> MGDHSQKDSPEDFIINRLSQALGIQKEKIKKSLETQQDDKGEVTNKDEFQGFIQQDNSTNILWVSGQSEKCTFYYGQLPPIDKFKKKGIAVIKLGLHKLTNENVAKDVVVVEITNNLLEHLNSVFNEIMSPVMQNPLNQQGWTDLVAKDLMEKFNNYVAQVYVLLGQIKGKTMLPLPSHKLTSSDTTPDKDKAHVFEGSIITWTKQIKNVLKLEPEQLLKYGNDPGPLAEIEFWQNKRDNLNLIDSQLKSVEVQNILHFLDNNKSTYTTPFTKLQAEVKKARLEANENYRYLFTLKDLFSKLQESQPSDFPTLYELFIPIMHTILLIYNKSKTYNQPPRLVVLIREICNAIISNAQAFVDKDTIFSLIDSKETTEACDKLQVTLDVCSKFKDAYFEYKAKAGGNWKLTSNALFVRLDSFLERCQDILHLTNTIVQFNKLEKIELGGTKGKTLTESIAQIFKEFEEAVQAFTSVSYDIMNIAEKKFDDDFYEFRSKIKELERRLASVITQGFDDYDTIYGRFKLLDNFEGLLTRPIIADELEKKHIVLLEMYKQDLKQVQSIFLEGKQFVDSMHENAPLFLNMPPIAGALTWCKSLRDRIQEPIEKLAQLGQGITEREEYKDVQKLYTSITKSIKDYEDQKILSWEKEVEDSSQDKLKQTLLCKDENDLIKVNFDPSLVRLLKEVKYFLLLRLEVPTTAKDIYTKAETYRTQIVALDMIVDNYNHIKTCLLPVEEPLVKKKIQDMEEEVKPGIEEIRWKSTNIDQFISKSKSIVDQLFETVNKMKDSLQKIHKSLANFNVKIIERKNRPMSPDDYDQFLKAIFSNKLTIVKDNGNQIQKLVKEVLDAVKADKKQNSWKNYNDYVNVIVIEGISTAIQTALLHLNEQINPVFIKRNDISPLFDIRLELGQSGIQFDPEIGESSNQLTVRNTIRNWINDFFNIAGTIQRLDTTMPGDFLQEIRSFFEIKQCLAMITQNLEWIENECNQFRARFDTYSYLWTEDEQISFNRFLDENEPKDEDGKGGDDDEGENTEKQNPLLKGCRAKIPNLDLFDEKITHLKAIQQEISRIKTPEDISWLRINLQPMKTALDARVTRWIRVYTDFLVNQFRTTQKNLLDFIEKTKDGIKKNPADHENLHDKKLLMSVMKVISDVKDVEPRREGIITRMKEMVTKLKKHNVPITEKGTDDPLQQIDNANSNFIEIYGRVFKVKADIIPLQAEETQNIKRDLDIFMKEVESFRKEFMQKLPFDYTESMGYENINNAYDTIMVYYHKLTAIEGRALEYNNLEKLFELQKSNYKQLKDCMNDLKNLKTMWDAIALIHFQYNDWKTKPWRQIKADILLDTNKTLGTQIKNLPKEIRNFKGYNVIVEKVKNMGTVLPLVSALHSEFMEDRHWSQLKQITGTVFDHNSLSFYFEDILALNLYKYENTVNEIVDVAQKEAKIEKKLKNIEQWWSKQVFEFTEYKETKTFASLDNMMEVLDQHSLDLMGMKSQGKYVEFFYDRVEDWREKLGRVDVVVNEWLKVQKNWKILYNIFLLSEDIRMQLPEDTKVFEGVDKEFKDMMSEVSANPSVVEACTIERRDVLVGWSQAIKKCEKALNDYLEQKKKSFPRFYFLSNQSLLTILSNGQNAPKVCEYLGDCFDGLKTLTFEPPANPAETSKVGIGMISKDDEKVPFSSKFICEGAVEHWLLNLEFRMRETLQEILEGAKNTADLWDSGDKPREEWVEGYNAQIALLTTTIVWTEDVGRAFEDLAGGSETAMKECQKLIEVRLENLIKKVRGDLHILERWKIINIITIDVHSRDVVEKFVIQKVSEAESFAWLSQLKFYWENKPDSDMHLRQTLRFPWEKDKNKNKCIIRIVDWFRFYSYEYIGNAIRLVITPLTDRCYITLTQALNLTMGGAPAGPAGTGKTETTKDLGRAIGIPVMVFNCSDQMNKDSMAQIFMGLSQSGAWGCFDEFNRISIEVLSVVSTQVKCVLDALKEKKTKFSFVEEGEIQLQDTVGFFITMNPGYAGRTELPENLKALFRSCAMVVPDLALICENMLM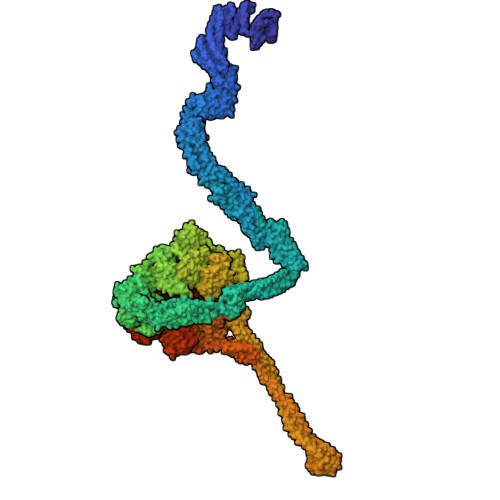SEGFTMARVLSRKFVSLYMLSRELLSKQKHYDWGLRAVKSVLRQAGKLKRGDPDMPEDPLLMRALRDFNMPKIVTDDKVIFRRLIGDLFPKLDPPTKQNPELKKIVQDTTKKDMGLVAEELFVTKVVQLAEILEVRHCCFVIGPPGSGKTCVWKTLIKSYINSGEDAEYDTLNPKAVTSDELFGAYTKTKEWKNGVIAVIMKNQVKNEEKYKATHMHKWSVLDGDIDPEWIESLNTVMDDNKVLTLVSNDRIFLTPQMRLIFEISNLRNATPATVSRAGVLFINETDIGWMPYMNSWLERSQINILKQQKEMANMPEYPVIDDVAKSVFYRCFQSYFEQNIDVHDKNRVRHICPMVDIAMIQTICTILDALLIQHLPKLKQMKEEDEKQALEAFFIFAGLWAIGGPVGGGQDDSKDMKEFNTVWKGAAKVKFPEQGLCYDYYYDINENKWNTWKVEDYLPNDQPLFSKIYVATIHTTRLRYMIDIHLQRRKPILFIGSAGTGKTAVVRDYLNSTRPEQVSHKTINFSSFTDSLALQKNIESMVEKKNGRNYGSATNKVLICFIDDFNMPYVDKYGTQSPIQLLRLILDYGSIFNREQLEERKFLQDLLFFGCLNQKSGSFTVDLRLQRNFSVFSMYTPSSDVIKTIFGSILNAHLSTIDDKAQKMAFKLVEATYFTFDKILKNTTAFAPSAKRFHYQFNFRELARVCEGICRTTPGQYSGGDQGKLVRLWAHEMKRTFEDRFIANEHVEFFRRYLTEAISKCIGEFPETENPIAEPLIFTGFVAAHQGLDQQYTQCTIPVLKRVLDDKLEEYNEVKAQMNLVLFQQAMEHVSRICRILDMPGNNALLVGVGGSGKQSLCRLSTFINGFEIDQLVVTASFTINDLRNNLQEIYKKIAKPNSIARVFMITDSQIKEEQFLIPINDMLNSGWIFDLFPKEDMDSLVSGVRNEAKGEGVDVNNLTALTSYFLDKIRKNLKVVLCFSPVGDTMRIRSRKFPGIINNTSIDWFHPWPHEALIDVAFRFLEEIEFPTEEIRQSISLNMAKVHSSIDTANEKFLKLERRYNYTTPKSFLELIDFYKKLLTEKRETIQRQIQRYEMGLNILAETQNKVQGLQEELKVKMVEVNKQREETDILIEKVGKESALAEEEQTIANAEEEKTNVAAAEAEKISKEATEALAEALPALRSAEAAVDCLKKPHVTEMKNLGSPPAGVIVTARVVLILFNQGITLNDPDEKVWKKAVTFMNNPQAFIDKVKSFDGENIEPNIIEQSNKIIQDPSKKFNEKDMAGQSYAASKLCAWAVNIVTFNKIFKQVKPLQDAQKQANEILEEKKKELAIVKQRVAELNARVNSLKRQLEEAEARKMIVEQDAARCQSRLSAAENLVNGLAGENKRWTQNVKFLKENIKSMIGDSLLASAFVSYIGAFSAKLRLELWKNTWLPDIIEKGIPITEGIEPLKILTTEAIKSKWKNEGLPADPMSLENAAIITACARWPLIIDPQLQGSTWIRGKQGENLTTISLSQPKWLGALTSSISSGRAVLIEGIQQEIDATLDPLLQRAVKKNGNQLQLEIGGDPIDYDPNFKLFLMTKLINPHFRPEIAAQCTIINFIVTESGLEEQFIAMVVNIEKNELEMAKQDLVKKQNEYAVTLDKLESDLLQSLSEADPATILDNTELIQNLDKTKKTTIEITEQQQKAKVTEAEINIQREHYRVVAAEGSMLYFLVISLSVMDHMYQYSLESFITFFFKAINRTTVRDENRIPTLILNIRQTIYQWISRGLFEKHKLIFLTLIVFRLMQKKIIDVAYEVAEMDFLIKCPARPGVENTLDWLPNISWDQIQGLINLEEFRNFAHQLEKEAPNRFKDWYNELQPEDQKLPLDWKRLDSMPFKKLLVLRCLRPDRMTISLNNFIRAVLPQGDAFVEMDQKLAFSEILESVINEDSESTIPIFFILSPGSDPVKEVEKIAKKKRIEPGKNFFNIALGQGQDEIARRRIEEGNKEGHWVMLQNIHLMPTWLIELEKILDSYSGEAGGGNSEFRLFLSAEPSTGIPIGILDRSIKLTNEPPAGLKANMKRAWTYFSKEEIEDKDPKIKSILFALCFFHSTLIERRRFGPKGWNMSYPFNMGDLRDSYLVMNRYMEQNQGGKVPFNDLIYIFGEIMYGGHIVDDWDRRLCNSYLFNTMHEQLFDELELFPYIEGKGLSFKVPGQNPYEKYIEHIETSLKQETPLAYGLHPNAEIGFRTDQCKTLFNTLLELMPKEQSRDEKSSDIKSSNEMASDLIKQLLEDSELKNKIFNMEEIKNKIDAENKGPYQNVFLQEIEYMNALLSEIVKDLEEIGQGLSGLLTVSENMEMIIESIALSRVPASWQKLAYPSKRGLQSWLANLFQRIEQLNIFRDDPYSIPRVVMISRFFNPQSFLTAIMQVISRAKAYELNKLYIQTEITKRSIEEIEGAAKEGAYVYGFILEGARWDYQLGQLEESKPKEMFSVLPVTYCKAIPLPPEGKEDKSLYQCPVYKTEDRGNTYVFTAQLKTRFPPRKWILAGVAIIMDVEGVSDEVKKDKK>GSHMEVVNMKAKEIIEFIETFAPKDLAIEGDNIGLQVGDNLDKEIKKLGIALDPSLSVIKKAEKEGVDFLFTHHPLLKDPIRNFTGVIYK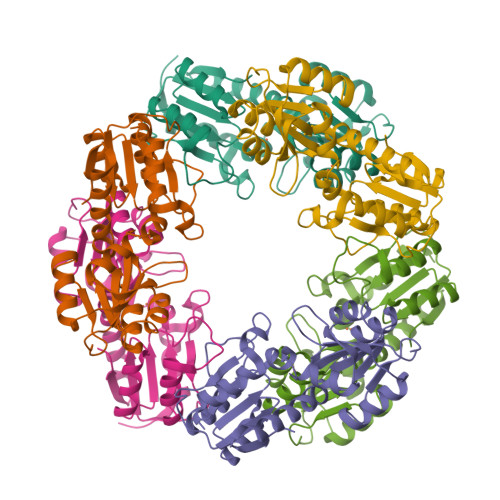KLKILMENDIILYSAHTNLDICKNGLNDALAELYNLENPKPLYDNGLGRVGIFKGSFEEFLEITKKYIHKNPIVVKSKEVDDNFKLAVLSGYGLSQSSIKYVAEKADVYLSGDLTHHSKILAEELGLVVVDATHYSTEVFGLKKFKEFLSSNLDLEIISLDF[6x]> GHMEDATLQEFPNAVNSFTPSVYKEVLKT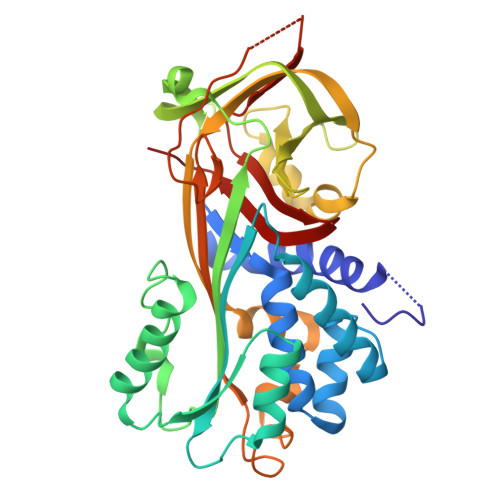EKANFLVSPFSAATLLALAQSGCRGDTAEEIRQVLHFVGDREKAEGAVKEVLSKLTNEEYTLHTANKIYVKTNFSVREEFQKIAVEVYGAQSENVDFSEKNDAAKLMNAWVEEQTQHKIQNLVDPEILNNLTRVVLINALYFNAKWLVPFPPFHTRKSDFHKSAKEVVQVDTMYLDEQYFNYYECHHLDAKLLELPFKGGASLTIVLSNQIEGLVSLESKIKRSFLPHNLTKQLVNVALPKFKIESTVDFKKVLKKLGVKKAFGDEADLSGIAGEKGDLVISNIVQKSFIDVSEEGVEAAAATYIPVILPEMALPDSPKQFIVDHPFIFYIKVKGMILFAGRVTTLN MODIFIED ACARBOSE HEXASACCHARIDE | C37 H63 N 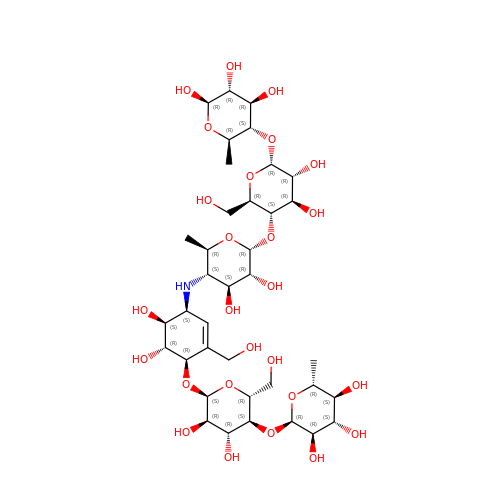O26 | YXELUDMUQSCWQW-HCVSURSQSA-N>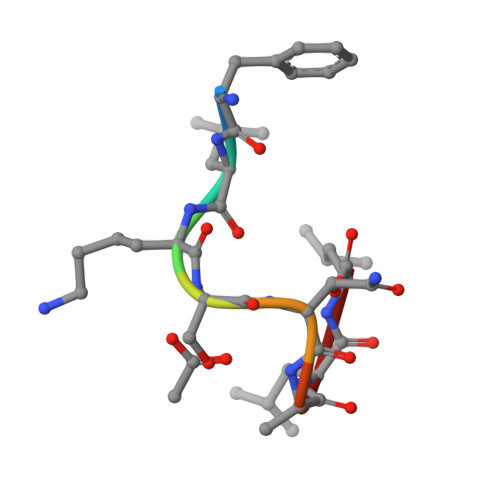FLKSXALL[2x]> SNAMLPVIAIVGRPNVGKSTLFNYLTKSRAALVADVPGVTRDRQYGETTIDSQRLLLVDTGGLVDTENKEVAPLAETQVEQAIDESDCILFLVDAKAGLVPADEIIAERLRKKGKKIFLAVNKADRARAAVVQSDFYKLGFGEPYVIAAASGRGVKDLMTQVLENLPEEKEVIEKEVGIKIAMIGRPNVGKSTLINRLLGEERVIVYDQPGTTRDSIYIPFARNDENYTLIDTAGIRR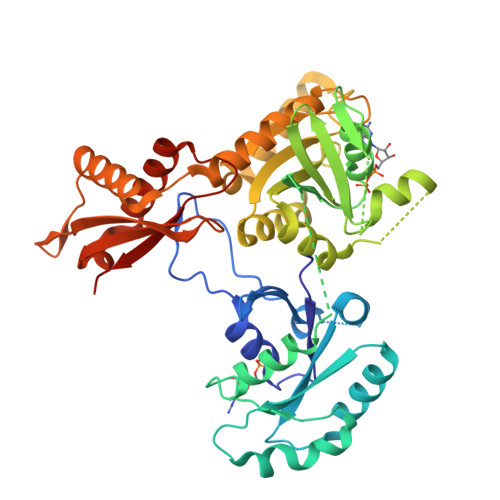RAKIQDYVEKFSMIKSLQAMHAADVVIFLLDARQGVTEQDLRLLNRIVEAGVSLIIAVNKWDGLNIEERDNVRNAIDRRMPFVDFARRYFISALHGTGVGKLFRAIQESYQSIQQELTTGQLTRALEKAVAEHEPPLVKGRRIRLRYAHLGARHPLTIVVHGKQTKSLPQSYSRYLANYFRKTFNFIGVPVHIKLKTDPNPYEGQEER>GPHMEDEAYFIAKEILATERTYLKDLEVITVWFRSVLIKEEAMPAALMALLFSNIDPVYEFHRGFLHEVEQRLALWEGPSSAHLKGDHQRIGDILLRNMRQLKEFTSYFQRHDEVLTELEKATKHCKKLEAVYKEFELQKVCYLPLN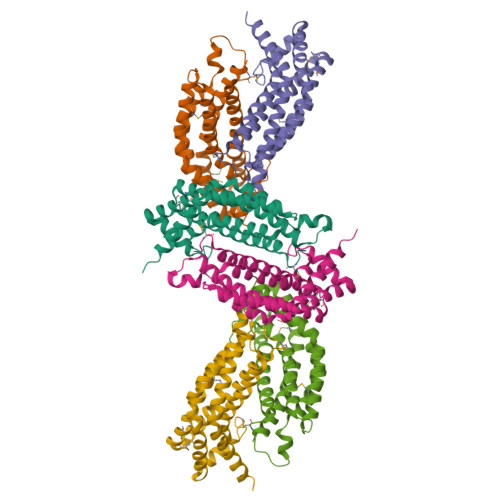TFLLKPVQRLVHYRLLLSRLCAHYSPGHRDYADCHEALKAITEVTTELQQSLTRLENLQKLTELQRDLVGV[9x]>[3x]MKVYIIDYHKDDPKRCTGKKLVKLKIAEFTRVGKGVVLDPFAQITLSNKD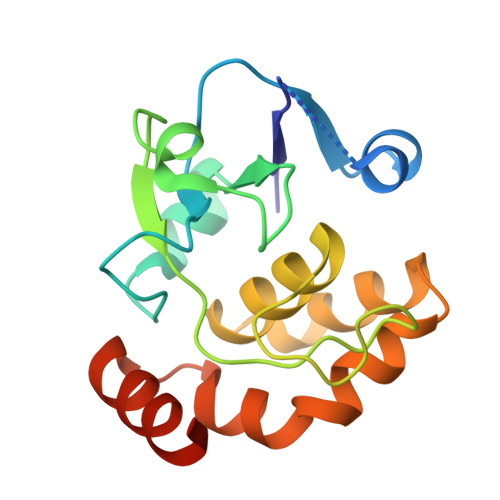KDIVRRIGITIVDTSWNNTSQSEFKNIRGEHRRIPILFAGNPIHYGIAYKLSSIEALIATLYIVDEVEEAIKLSNVVKWGHTFIELNKELLEAYKNKTEEDIKKIEREIIEKILEK5-phenyl-1H-1,2,3-triazole-4-carboxylic acid | C9 H7 N3 O2 | 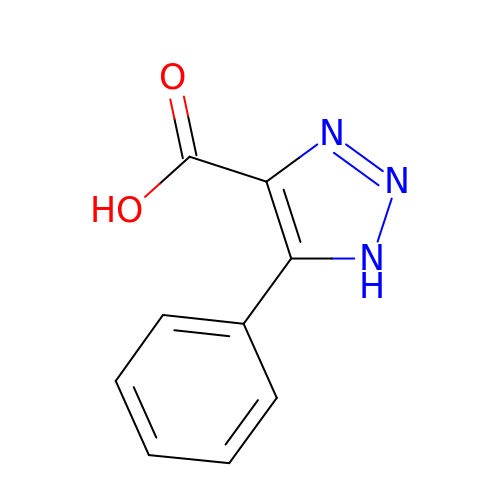KZVFXYXQNAYXFT-UHFFFAOYSA-N>[6x]MRKQLDELLDIKESARGGPDPDATRRQHDKGKLTARERIELLLDKDSFQEIEQLRRHRATGFGLEAKKPYTDGVITGWGTVHGRTVFVYAHDFRIFGGALGEAHAQKIHKLMDMAIAAGAPLVSLNDGAGARIQEGVTALAGYGGIFQRNTRASGVIPQISVMLGPCAGGAAYSPALTDFVFMVRGTSQMFITGPDVVRAVTGEEIGQEGLGGADVHSRTSGVAHFAYDDEETCLEEVRFLLSMLPANNRESAPAVPCDDPADRRGQALYDLVPADGNRPYDMRAVIEEIVDDGTHLEVHERWATNVICTLARLDGKVVGIVANQPQSLA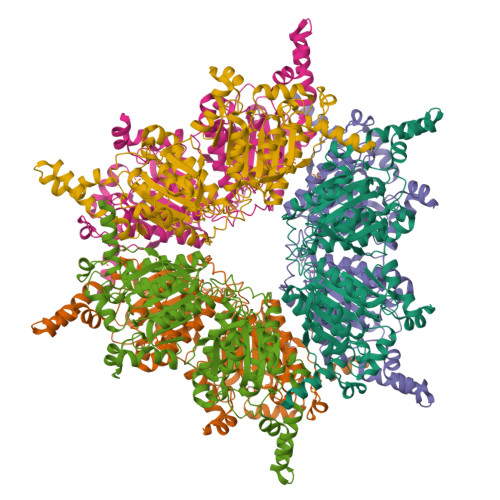GVLDIAASEKAASFVQTCDSFNIPLVTLLDVPGFLPGVDQEHNGIIRHGAKLLYAYCNATVPRISLVLRKAYGGAYIVMDSRSIGADLALAWPTNEIAVMGAEGAAGVIFRRDINAADDPEAVRRQRVEEYKAELMHPYYAAERGLVDDVIDPADTREVLIRGLAMLRTKHADLPMRKHGNPPQ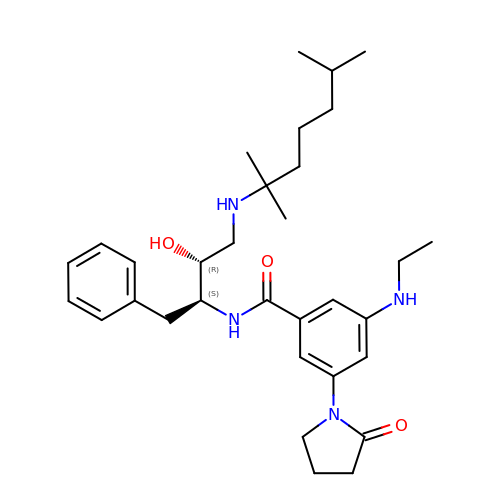N-{(1S,2R)-1-benzyl-2-hydroxy-3-[(1,1,5-trimethylhexyl)amino]propyl}-3-(ethylamino)-5-(2-oxopyrrolidin-1-yl)benzamide | C32 H48 N4 O3 | BNTVCVCCNARYIP-URLMMPGGSA-N> AENSDFYLPGDYLLGGLFSLHANMKGIVHLNFLQVPMCKEYEVKVIGYNLMQAMRFAVEEINNDSSLLPGVLLGYEIVDVCYISNNVQPVLYFLAHEDNLLPIQEDYSNYSSRVVAVIGPDNSESVMTVANFLSLFLLPQITYSAISDELRDKVRFPALLRTTPSADHHIEAMVQLMLHFRWNWIIVLVSNDTYGRDNGQLLGERVARRGICIAFQETLPTLQPNQNMTSEERQRLVTIVDKLQQSTARVVVVFS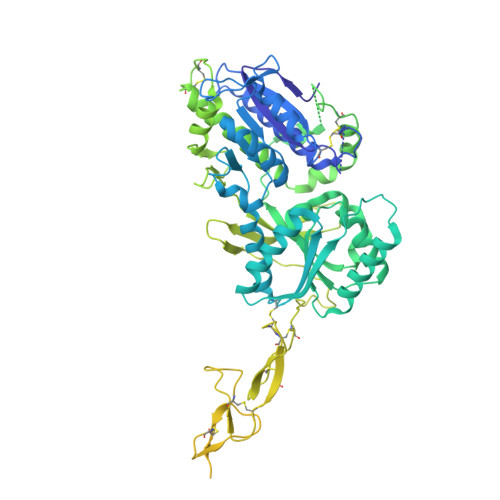PDLTLYHFFNEVLRQNFTGAVWIASESWAIDPVLHNLTELRHLGTFLGITIQSVPIPGFSEFREWGPQAGPPPLSRTSQSYTCNQECDNCLNATLSFNTILRLSGERVVYSVYSAVYAVAHALHSLLGCDKSTCTKRVVYPWQLLEEIWKVNFTLLDHQIFFDPQGDVALHLEIVQWQWDRSQNPFQSVASYYPLQRQLKNIQDISWHTINNTIPMSMCSKRCQSGQKKKPVGIHVCCFECIDCLPGTFLNHTEDEYECQACPNNEWSYQSETSCFKRQLVFLEWHEAPTIAVALLAALGFLSTLAILVIFWRHFQTPIVRSAGGPMCFLMLTLLLVAYMVVPVYVGPPKVSTCLCRQALFPLCFTICISCIAVRSFQIVCAFKMASRFPRAYSYWVRYQGPYVSMAFITVLKMVIVVIGMLATGLSPTTRTDPDDPKITIVSCNPNYRNSLLFNTSLDLLLSVVGFSFAYMGKELPTNYNEAKFITLSMTFYFTSSVSLCTFMSAYSGVLVTIVDLLVTVLNLLAISLGYFGPKCYMILFYPERNTPAYFNSMIQGYTMRRD> TWGVSSPKNVQGLSGSCLLIPCIFSYPADVPVSNGITAIWYYDYSGKRQVVIHSGDPKLVDKRF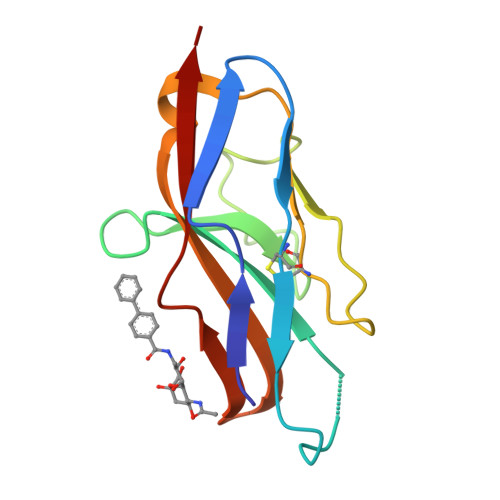RGRAELMGNMDHKVCNLLLKDLKPEDSGTYNFRFEISDSNRWLDVKGTTVTVTTD> SPLKPRNYQLELALPAKKGKNTIICAPTGCGKTFVSLLICEHHLKKFPCGQKGKVVFFANQIPVYEQQATVFSRYFERLGYNIASISGATSDSVSVQHIIEDNDIIILTPQILVNNL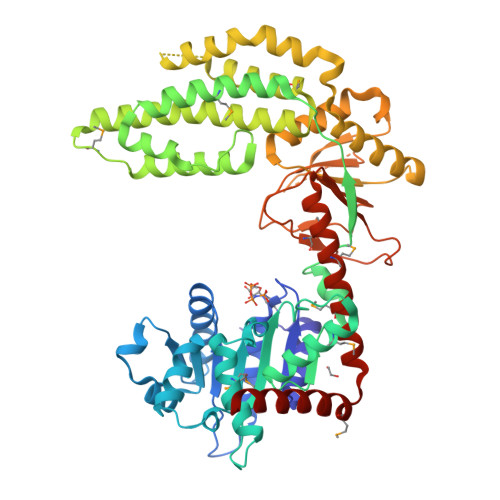NNGAIPSLSVFTLMIFDECHNTSKNHPYNQIMFRYLDHKLGESRDPLPQVVGLTASVGVGDAKTAEEAMQHICKLCAALDASVIATVRDNVAELEQVVYKPQKISRKVASRTSNTFKCIISQLMKETEKLAKDVSEELGKLFQIQNREFGTQKYEQWIVGVHKACSVFQMADKEEESRVCKALFLYTSHLRKYNDALIISEDAQMTDALNYLKAFFHDVREAAFDETERELTRRFEEKLEELEKVSRDPSNENPKLRDLYLVLQEEYHLKPETKTILFVKTRALVDALKKWIEENPALSFLKPGILTGRGRTNRATGMTLPAQKCVLEAFRASGDNNILIATSVADEGIDIAECNLVILYEYVGNVIKMIQTRGRGRARDSKCFLLTSSADVIEKEKANMIKEKIMNESILRLQTWDEMKFGKTVHRIQVNEKLLRDS> KYNLKMGMTAGTSQNEYKAAEVFAKELKKRSNGEIELKLYPNAQLGKDDLAMMQQLEGGALDFTFAETGRFSTFFPEAEVFTLPYMIKDFNHMKKAVNTKFGKDLFKKVHDKKGMTVLAQAYNGTRQTTSNKAIKSLADMKGMKLRVPGAAANLAYAKYTEAAPTPMAFSEVYLALQTNAVDGQENPLSTIKAQKFYEVQKYLAMTNHILNDQLYLVSNITMEELPENLQKVVKESAEVAAEYHTKLFMDEEKSLKDFFKSKGVTITEPNLVDFKKAMKPFYDEYIKKNGKVGENAIKAIEAVRLEHHHHHH

The first step of this process is the transport of sialic acid to the cytoplasm, which often takes place using a tripartite ATP-independent transport system consisting of a periplasmic binding protein and a membrane transporter. In this paper, the structural characterization of periplasmic binding proteins from the pathogenic bacteria Fusobacterium nucleatum, Pasteurella multocida and Vibrio cholerae and their thermodynamic characterization are reported. The structure and the thermodynamics of the binding of sugars suggest that all of these proteins have a very well conserved binding pocket and similar binding affinities. While the C1 carboxylate has been identified as the primary binding site, a second conserved hydrogen-bonding network is involved in the initiation and stabilization of the conformational states.

Pm-SiaP and Fn-SiaP were crystallized together with Neu5Ac. Their structures were determined to 1.57 and 2.5 Å resolution, respectively. The structure of Pm-SiaP was refined to an R factor of 0.17 and a free R factor of 0.20, and that of Fn-SiaP was refined to an R factor of 0.21 and a free R factor of 0.25. All three proteins (Pm-SiaP, Fn-SiaP and Hi-SiaP) have very similar structures, distinguished by two domains on either side of a well defined pocket, within which Neu5Ac binds. In all of the Neu5Ac-bound structures, a consistent pattern was seen in how Neu5Ac interacts with four of the residues within the pocket. Using Fn-SiaP as an example, Arg126 interacts with one of the O atoms of the carboxylate group at the C1 position and the O2 of Neu5Ac to form a second salt bridge. Asn186 interacts with O2 of Neu5Ac, and Asp50 interacts with O7. Similar inter­actions between these four residues and Neu5Ac exist in Hi-SiaP and Pm-SiaP, with minor differences in sequence numbering (e.g. Arg127 and Arg147 are involved in the first two interactions in Hi-SiaP), as also seen previously. There was one interaction seen in Hi-SiaP (between Asn10 and O10 of Neu5Ac) that was not evident in Fn-SiaP and Pm-SiaP. The binding affinities of Fn-SiaP and Pm-SiaP to Neu5Ac are 45.5 and 19.7 nM, respectively.>NTKYNKEFLLYLAGFVDGDGSIIAQIKPNQSYKFKHQLSLTFQVTQKTQRRWFLDKLVDEIGVGYVRDRGSVSNYILSEIKPLHNFLTQLQPFLKLKQKQANLVLKIIEQLPSAKESPDKFLEVCTWVDQIAALNDSKTRKTTSETVRAVLD[2x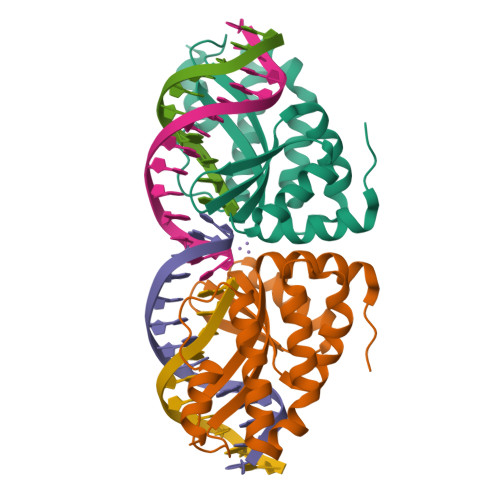]>MQGVNIYNISAGTSVDLAAPVTTGDIVTFFSSALNLNAGAGNPNNTTANLFAENGAYLLHIAFRLQENVIIFNSRQPDGPWLVEQRVSDVANQFAGIDGKAMVTVFDHGDKYQVVINEKTVIQYTKQISGLTSSLSYNATEETSIFSTVVEAVTYTGLALE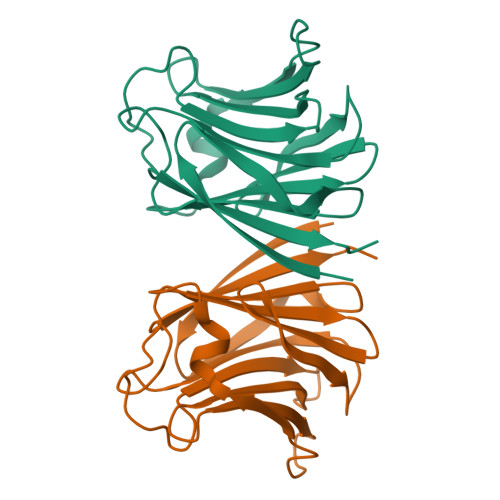HHHHHH[2x]> GCCSHPAC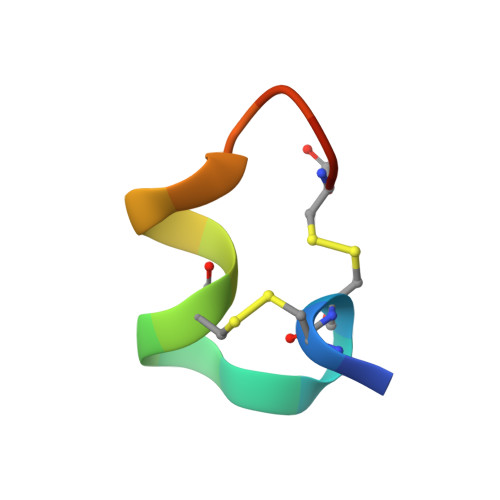NVDHPEICX> GPGSMARERTFLMVKPDGVQRGLVGEIISRFERRGFKLVAMKFFVPSKNLVEE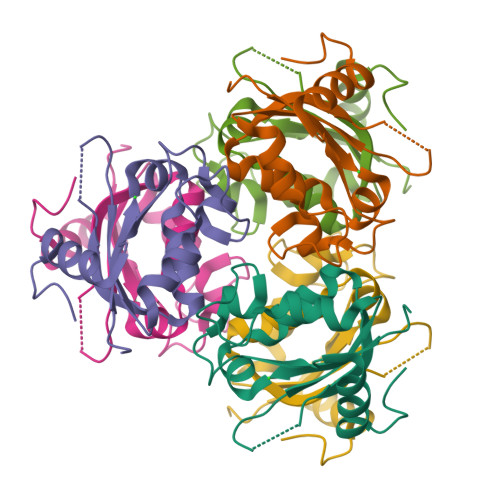HYKEHAARPFFAGLCKFLSSGPVCAMVWEGANVVSISRTMMGVTKPAESAPGTIRGDFGIDVGRNIIHGSANLDDAAREIALWFKPEEVASWSCSLESHIYE> 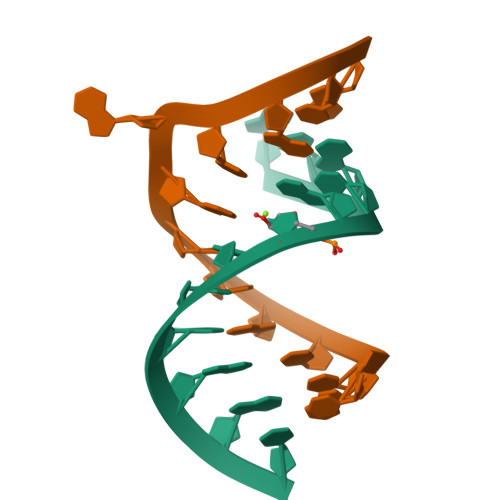GCGCGUAGUAGC;> CGCUACUGACGCG>[8x]MAFYKREMFDPAEKYKMDHRRRGIALIFNHERFFWHLTLPERRGTCADRDNLTRRFSDLGFEVKCFNDLKAEELLLKIHEVSTVSHADADCFVCVFLSHGEGNHIYAYDAKIEIQTLTGLFKGDKCHSLVGKPKIFIIQACRGNQHDVPVIPLDVVDNQTEKLDTNITEVDAASVYTLPAGADFLMCYSVAEGYYSHRETVNGSWYIQDLCEMLGKYGSSLEFTELLTL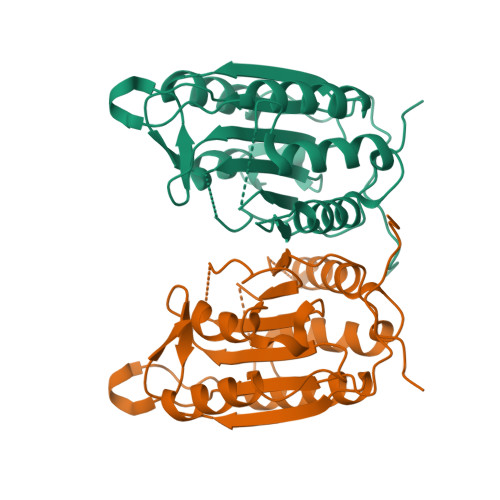VNRKVEQRRVDFCKDPSAIGKKQVPCFASMLTKKLHFFPKSNLEHHHHHH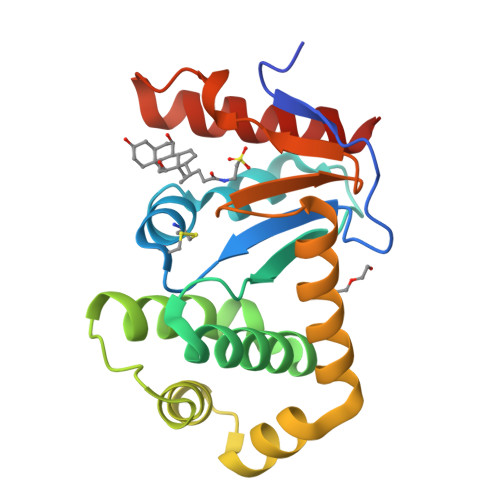> AQYEDGKQYTTLEKPVAGAPQVLEFFSFFCPHCYQFEEVLHISDNVKKKLPEGVKMTKYHVNFMGGDLGKDLTQAWAVAMALGVEDKVTVPLFEGVQKTQTIRSASDIRDVFINAGIKGEEYDAAWNSFVVKSLVAQQEKAAADVQLRGVPAMFVNGKYQLNPQGMDTSNMDVFVQQYADTVKYLSEKK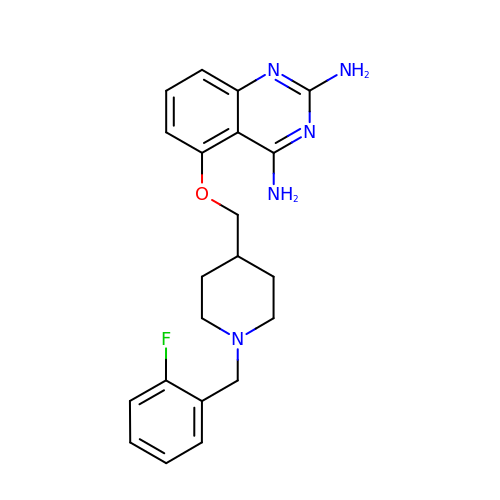5-{[1-(2-fluorobenzyl)piperidin-4-yl]methoxy}quinazoline-2,4-diamine | C21 H24 F N5 O | GYKIQIOWVKCVBP-UHFFFAOYSA-N>MTMASVPASRYLTDMTLEEMSRDWSMLIPKQKVAGPLCIRMDQAIMDKNIILKANFSVIFDRLETLILLRAFTEEGAIVGEISPLPSLPGHTAEDVKNAVGVLIGGLEWNDNTVRVSETLQRFAWRSSNENGRPPLTPKQKREMAGTIRSEV[2x]

During infection the influenza A virus NS1 protein participates in multiple protein-RNA and protein-protein interactions to perform a plethora of functions. The N-terminal 73 amino-acid residues of NS1 form a symmetrical homodimeric RNA-binding domain (RBD), which is connected to the central effector domain (ED; residues 86-204) via an inter-domain linker. Present models of the tertiary and quaternary structures of NS1 indicate that the protein possesses two globular domains, each capable of forming independent homodimeric interactions. Our bioinformatic analyses indicate that the N-terminal RBD forms a very stable homodimer, while the predominant and ubiquitous helix-helix contacts between C-terminal EDs bear many similarities with weak transient interfaces.

In contrast, several possible ED homodimer interfaces have been proposed based upon crystal structures obtained using NS1 proteins from various strains. While the helix-helix interface appears to be the only dimeric form of NS1 ED consistently observed in all crystal structures, it remains possible that other dimeric states (such as the strand-strand dimer) contribute to dimerization in solution. Although the helix-helix dimer interface is shared by all structures of the NS1 ED, and may have some biological role in that RNA-binding activity of NS1 is affected by its disruption, we noted that in all helix-helix structures the arrangement of the two ED monomers differs markedly relative to one another. However, at this same concentration we routinely observe complete dimerization of the PR8 and Alb/76 NS1 EDs. A key aspect of our functional model is the instability and flexibility of the NS1 ED helix-helix dimer, which seems weak and transient in vitro, but may be slightly more stable in the context of the full-length protein, or become more permanent in the presence of certain binding partners. ED dimer flexibility is likely permitted by the presence of several glycine residues at the homodimer interface (a putative GxxxG protein-protein interaction motif) that allow the two helices to rotate easily relative to one another.> MKPTYEILGQMDETFILVKDSEYLYFVDQHLLEERINYEKLKDENLACRISVKAGQKLSEEKIRELIKTWRNLENPHVCPHGRPIYYKIPLREIYEKVGRNY

MutLs, with a few exceptions, are endonucleases that incise the error-containing (i.e., newly synthesized) strand of the mismatched duplex. Prokaryotic MutL endonucleases and the endonuclease subunits of eukaryotic MutL homologs include two domains: the N-terminal ATPase domain and the C-terminal endonuclease domain (CTD). The dimerization subdomain contains the metal-binding sites, in which multiple zinc ions are coordinated by the residues from highly conserved motifs: DQHAX2EX4E, ACR, and CPHGRP (underlined residues coordinate the zinc ions). Here, we solved the crystal structure of the endonuclease domain of Aquifex aeolicus MutL in the manganese- or cadmium-bound form, revealing that these metals compete with zinc at the same sites.

In order to explore this possibility, we performed crystal structure analysis of the aqMutL CTD complexed with manganese ions. The aqMutL CTD, which is purified as the zinc-bound form, was incubated with the buffer solution containing 2 mM manganese ion at 70°C for 24 h. The protein was concentrated and crystallized in the presence of a 50 mM manganese ion. The crystal structure was solved with manganese single-wavelength anomalous dispersion phasing. Peaks of electron density in the anomalous diffraction map calculated from data collected at a wavelength of 1.8900 Å were clearly observed at the M1, M2, and M3 sites of the aqMutL CTD at 100% occupancy. The overall structure of the manganese-bound form was almost identical to that of the zinc-bound form; the root-mean-square deviation between the two structures was 0.1 Å. No peak of electron density in the anomalous diffraction map was observed around Asp351 of the DQHAX2EX4E motif. Thus, it was confirmed that manganese ions bind to the same sites of aqMutL as zinc ions. The electron density of the guanidino group of Arg406 was also missing in the manganese-bound form of the aqMutL CTD. Likewise, the position of the α4 helix, the structure of Arg406, and the quaternary structure of the manganese-bound form were the same as those in the zinc-bound form (respectively).> MTKYKYTVEESERFNKHGIDLTVYGQVDPSATVVRVSVERGHFQEFFNVRSSYTYYVVSGQGVFYLNSEAVPAGATDLITVPPNTRIHYFGSMEMVLTVAPAFNEQDERHVRFISESESPY

In pacidamycin 3, biosynthesis the 3′‐deoxy moiety is mediated by Pac13, an enzyme found to catalyze the key dehydration of uridine‐5′‐aldehyde 1 to form 3′‐deoxy‐3′,4′‐didehydrouridine‐5′‐aldehyde 2. In stark contrast to most characterised dehydratases, Pac13 is small (121 aa), monomeric, co‐factor independent and utilises a non‐activated nucleoside, rather than a free monosaccharide, as a substrate. Pac13 is the only monomeric, metal‐free cupin dehydratase characterised to date. We demonstrate here that the reaction most likely proceeds via an E1Cb mechanism, with H42 acting as an active site base, however, unlike many other dehydratases, no metal or cofactor is required for activity.

Solution of the structure required the preparation of the seleno‐methionine derivative (SeMet‐Pac13) and demonstrated that the enzyme was indeed a cupin.> QIPASEQETLVRPKPLLLKLLKSVGAQKDTYTMKEVLFYLGQYIMT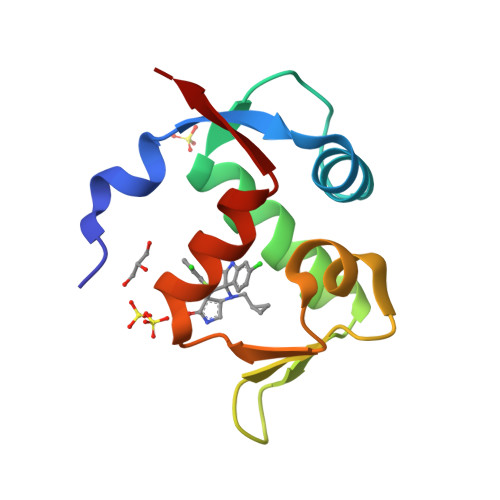KRLYDEKQQHIVYCSNDLLGDLFGVPSFSVKEHRKIYTMIYRNLVVVN[(1R,2R,3S,4S,5R)-2,3,4,5-TETRAHYDROXYCYCLOHEXYL]METHYL DIHYDROGEN PHOSPHATE | C7 H15 O8 P | 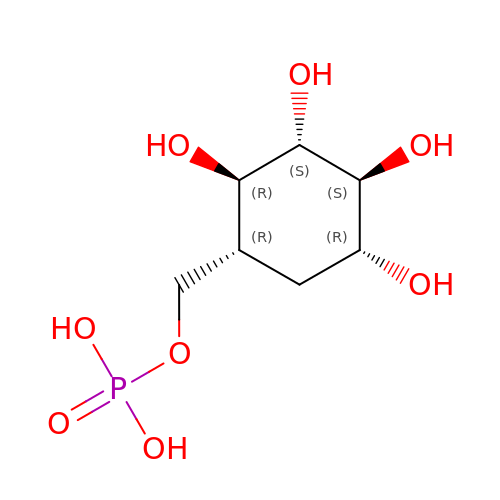FPLZFJHCPYNBEO-OVHBTUCOSA-N> PATGEKKECWSWESYLEEQKAITAPVSLFQDSQ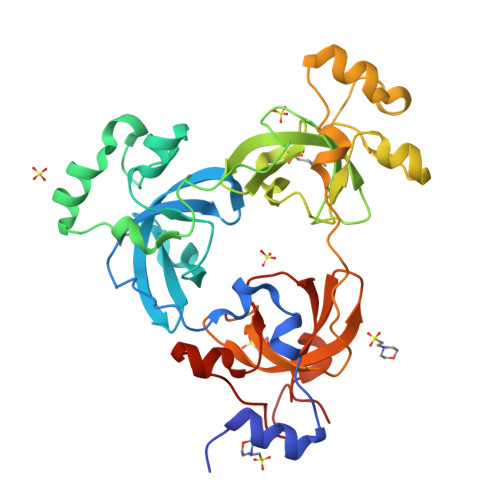AVTHNKNGFKLGMKLEGIDPQHPSMYFILTVAEVCGYRLRLHFDGYSECHDFWVNANSPDIHPAGWFEKTGHKLQPPKGYKEEEFSWSQYLRSTRAQAAPKHLFVSQSHSPPPLGFQVGMKLEAVDRMNPSLVCVASVTDVVDSRFLVHFDNWDDTYDYWCDPSSPYIHPVGWCQKQGKPLTPPQDYPDPDNFCWEKYLEETGASAVPTWAFKVRPPHSFLVNMKLEAVDRRNPALIRVASVEDVEDHRIKIHFDGWSHGYDFWIDADHPDIHPAGWCSKTGHPLQPPLGPREPSSAS>[2x]MKRVLSGIQPSGEIHIGN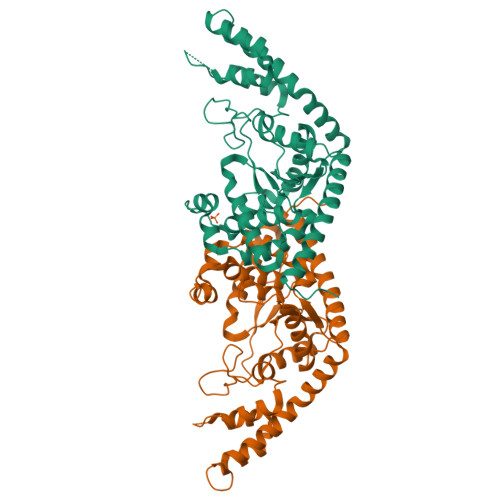YLGAIKQWVAIGEKLGRDAFFCIVDYHALTNPLAYDPSTLAQRTFEAALVNIAAGLDPEKVTLFVQSHVPEHTELSWVFTTLTPLGDLTRMTQFKDKASKQETVWSGLLMYPVLQAADILIYKADTVPVGEDQVQHIELTREIARRFNHLFGETFPEPQALLNPEAPRVPGIDGKAKMSKSLGNTIGLLEPEESIWQKIQHLPDDPQRIRLSDPGDPERTILFTYLSYFAPKDLVEALKEEYRKAGVGTYVVKRILFDHLMEALRPIRERAEALKKDPDYVMDALLEGAKRARAVAQATMEEVREKVGLLLPRKRPVLR> MSYQVLARKWRPQTFADVVGQEHVLTALANGLSLGRIHHAYLFSGTRGVGKTSIARLLAKGLNCETGITATPCGVCDNCREIEQGRFVDLIEIDAASRTKVEDTRDLLDNVQYAPARGRFKVYLIDEVHMLSRHSFNALLKTLEEPPEHVKFLLATTDPQKLPVTILSRCLQFHLKALDVEQIRHQLEHILNEEHIAHEPRALQLLARAAEGSLRDALSLTDQAIASGDGQVSTQAVSAMLGTLDDDQALSLVEAMVEANGERVMALINEAAARG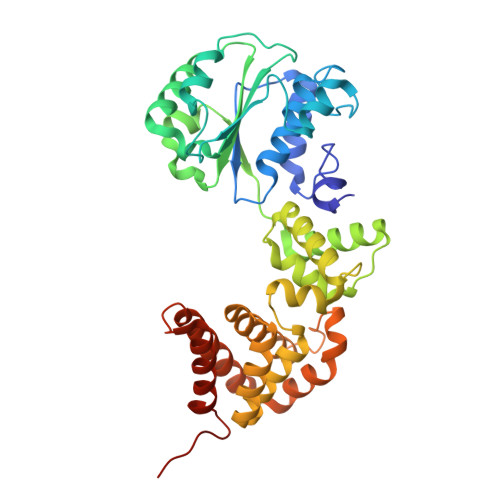IEWEALLVEMLGLLHRIAMVQLSPAALGNDMAAIELRMRELARTIPPTDIQLYYQTLLIGRKELPYAPDRRMGVEMTLLRALAFHPRMPLPEPEVPRQ>MKFLVNVALVFMVVYISYIYADPVLPKPLNAPNVIDTGHNFAVINISSEPYFGDGPIKSKKLLYKPVNHYEAWQHIQVTNEIVTLNYLEPRTEYELCVQLVRRGEGGEGHPGPVRRFTTASIGLPPPRGLNLLPKSQTTLNLTWQPIFPSSEDDFYVEVERRSVQKSDQQNIKVPGNLTSVLLNNLHPREQYVVRARVNTKAQGEWSEDLTAWTLSDILPPQPENIKISNI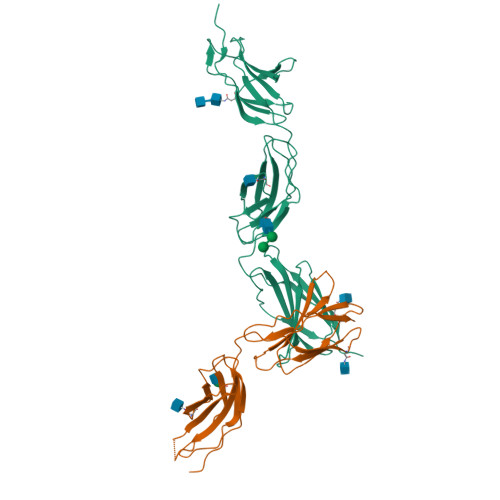THSSAVISWTILDGYSISSITIRYKVQGKNEDQHVDVKIKNATITQYQLKGLEPETAYQVDIFAENNIGSSNPAFSHELVTLPESQAPADLGIEGRHHHHHH[2x]>ITRKLILAGNWKMHKTISEAKKFVSLLVNELHDVKEFEIVVCPPFTALSEVGEILS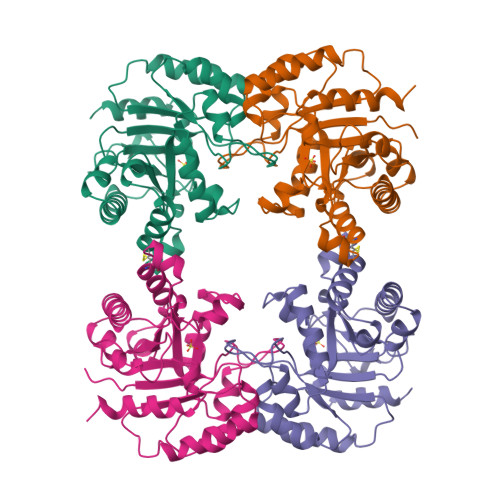GRNIKLGAQNVFYEDQGAFTGEISPLMLQEIGVEYVIVGHSERRRIFKEDDEFINRKVKAVLEKGMTPILCVGETLEEREKGLTFCVVEKQVREGFYGLDKEEAKRVVIAYEPVWAIGTGRVATPQQAQEVHAFIRKLLSEMYDEETAGSIRILYGGSIKPDNFLGLIVQKDIDGGLVGGASLKESFIELARIMRGVIS[2x]Astragalin | 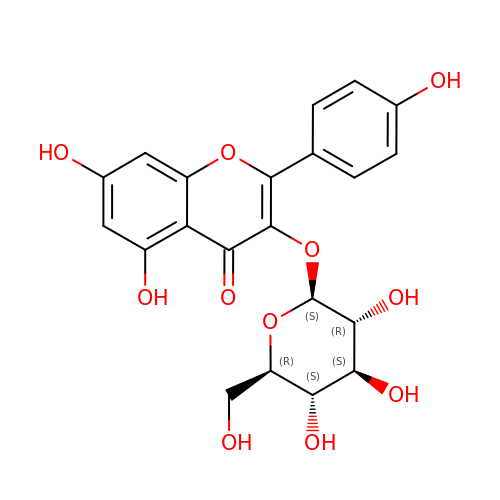C21 H20 O11 | JPUKWEQWGBDDQB-QSOFNFLRSA-N1-(phenylmethyl)-4-pyrrol-1-yl-piperidine | C16 H20 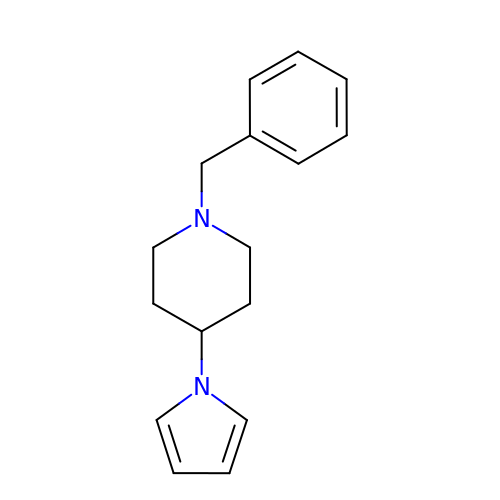N2 | UPRFZLANTXURKF-UHFFFAOYSA-N>SMRVKAAQAGRQSSAKRHLAEQFAVGEIITDMAAAAWKVGLPIGQGGFGCIYLADMNSSESVGSDAPCVVKVEPSDNGPLFTELKFYQRAAKPEQIQKWIRTRKLKYLGVPKYWGSGLHDKNGKSYRFMIMDRFGSDLQKIYEANAKRFSRKTVLQLSLRILDILEYIHEHEYVHGDIKASNLLLNYKNPDQVYLVDYGLAYRYCPEGVHKAYAADPKRCHDGTIEFTSIDAHNGVAPSRRGDLEILGYCMIQWLTGHLPWEDNLKDPKYVRDSKIRYRENIASLMDKCFPAANAPGEIAKYMETVKLLDYTEKPLYENLRDILLQGLKAIGSKDDGKLDLSVVENGGLK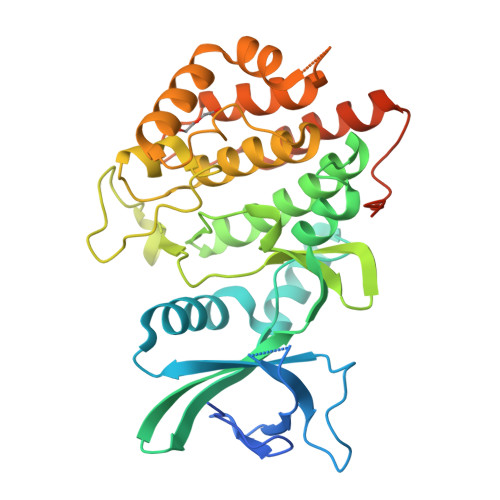AKTITKKRAAEIEE[4x]The m6A “writer” consists of the catalytic subunit m6A-METTL complex (MAC) and the regulatory subunit m6A-METTL-associated complex (MACOM), the latter being essential for enzymatic activity. Deposition of m6A onto RNAs is achieved by the m6A methyltransferase complex (m6A writer), a large holocomplex of ~1000 kDa in size that contains methyltransferase-like 3 and 14 (METTL3/14), Wilms’ tumor 1-associated protein (WTAP), KIAA1429 (VIRMA), Zinc finger CCCH domain-containing protein 13 (ZC3H13), RNA binding motif protein 15/15 paralog (RBM15/15B), and E3 ubiquitin ligase CBLL1 (HAKAI). Here, we report the cryo-electron microscopy (cryo-EM) structures of MACOM at a 3.0-Å resolution, uncovering that WTAP and VIRMA form the core structure of MACOM and that ZC3H13 stretches the conformation by binding VIRMA. Our cryo-EM structure reveals that WTAP forms a homodimer, with each monomer consisting of four tandem helices (H1–H4/H1’–H4’ with coiled-coil interactions) and three linkers (L1–L3/L1’–L3’).

To understand the structural basis of the MACOM function, we determined the 3.0-Å resolution structures of the HWVZ and HWV complexes using single-particle cryo-EM analysis. To our surprise, in the cryo-EM structure of the HWVZ complex, only three components (WTAP, VIRMA, and ZC3H13) can be found, while HAKAI is missing, although it is present in the SDS-PAGE analysis, indicating the high flexibility of HAKAI. Human WTAP (residues 64–247), VIRMA (residues 334–1585), and ZC3H13 (residues 1492–1643) form a compact structure shaped like a “warhorse” that represents the core of human MACOM. Unlike WTAP and VIRMA that form saddle- and horse-like conformations, respectively, the C-terminal fragment of ZC3H13 is only one-tenth of its full length and contains eight α-helices, but it does not exhibit a rigid conformation. Instead, it attaches to the Belly, Chest, and Neck domains of VIRMA and functions like a barding to protect the horse body (Supplementary informaiton, Video S1). Therefore, this fragment of ZC3H13 is called the Barding domain. The Barding domain of ZC3H13 has a strong interaction with VIRMA, and the interface is ~4435 Å2, involving seven salt bridges and 19 hydrogen bonds. In contrast, the interaction between the Barding domain and WTAP is weak, with an interface area of ~256 Å2 in which highly conserved residues R1512 and F1521 of the first α-helix of the Barding domain form salt bridges and hydrophobic interactions with D206 and F207 in H4 of WTAP-a, respectively. Our structural study shows that ZC3H13 uses its C-terminal Barding domain to interact with VIRMA and induce the conformational change of MACOM.

> MAVDSAMELLFLDTFKHPSAEQSSHIDVVRFPCVVYINEVRVIPPGVRAHSSLPDNRAYGETSPHTFQLDLFFNNVSKPSAPVFDRLGSLEYDENTSIIFRPNSKVNTDGLVLRGWYNCLTLAIYGSVDRVISHDRDSPPPPPPPPPPPQPQPSLKRNPKHADGEKEDQFNGSPPRPQPRGPRTPPGPPPPDDDEDDPVPLPVSGDKEEDAPHREDYFEPISPDRNSVPQEGQYSDEGEVEEEQQEEGEEDEDDVDVEEEEDEDEDDRRTVDSIPEEEEEDEEEEGEEDEEGEGDDGYEQISSDEDGIADLERETFKYPNFDVEYTAEDLASVPPMTYDPYDRELVPLLYFSCPYKTTFEIEISRMKDQGPDKENSGAIEASVKLTELLDLYREDRGAKWVTALEEIPSLIIKGLSYLQLKNTKQDSLGQLVDWTMQALNLQVALRQPIALNVRQLKAGTKLVSSLAECGAQGVTGLLQAGVISGLFELLFADHVSSSLKLNAFKALDSVISMTEGMEAFLRGRQNEKSGYQKLLELILLDQTVRVVTAGSAILQKCHFYEVLSEIKRLGDHLAEKTSSLPNHSEPDHDTDAGLERTNPEYENEVEASMDMDLLESSNISEGEIERLINLLEEVFHLMETAPHTMIQQPVKSFPTMARITGPPERDDPYPVLFRYLHSHHFLELVTLLLSIPVTSAHPGVLQATKDVLKFLAQSQKGLLFFMSEYEATNLLIRALCHFYDQDEEEGLQSDGVIDDAFALWLQDSTQTLQCITELFSHFQRCTASEETDHSDLLGTLHNLYLITFNPVGRSAVGHVFSLEKNLQSLITLMEYYSKEALGDSKSKKSVAYNYACILILVVVQSSSDVQMLEQHAASLLKLCKADENNAKLQELGKWLEPLKNLRFEINCIPNLIEYVKQNIDNLMTPEGVGLTTALRVLCNVACPPPPVEGQQKDLKWNLAVIQLFSAEGMDTFIRVLQKLNSILTQPWRLHVNMGTTLHRVTTISMARCTLTLLKTMLTELLRGGSFEFKDMRVPSALVTLHMLLCSIPLSGRLDSDEQKIQNDIIDILLTFTQGVNEKLTISEETLANNTWSLMLKEVLSSILKVPEGFFSGLILLSELLPLPLPMQTTQVIEPHDISVALNTRKLWSMHLHVQAKLLQEIVRSFSGTTCQPIQHMLRRICVQLCDLASPTALLIMRTVLDLIVEDLQSTSEDKEKQYTSQTTRLLALLDALASHKACKLAILHLINGTIKGDERYAEIFQDLLALVRSPGDSVIRQQCVEYVTSILQSLCDQDIALILPSSSEGSISELEQLSNSLPNKELMTSICDCLLATLANSESSYNCLLTCVRTMMFLAEHDYGLFHLKSSLRKNSSALHSLLKRVVSTFSKDTGELASSFLEFMRQILNSDTIGCCGDDNGLMEVEGAHTSRTMSINAAELKQLLQSKEESPENLFLELEKLVLEHSKDDDNLDSLLDSVVGLKQMLESSGDPLPLSDQDVEPVLSAPESLQNLFNNRTAYVLADVMDDQLKSMWFTPFQAEEIDTDLDLVKVDLIELSEKCCSDFDLHSELERSFLSEPSSPGRTKTTKGFKLGKHKHETFITSSGKSEYIEPAKRAHVVPPPRGRGRGGFGQGIRPHDIFRQRKQNTSRPPSMHVDDFVAAESKEVVPQDGIPPPKRPLKVSQKISSRGGFSGNRGGRGAFHSQNRFFTPPASKGNYSRREGTRGSSWSAQNTPRGNYNESRGGQSNFNRGPLPPLRPLSSTGYRPSPRDRASRGRGGLGPSWASANSGSGGSRGKFVSGGSGRGRHVRSFTR;> PVATATATTVPATLAATTAAAATSFSTSAITISTSATPTNTTNNTFANEDSHRKCHRTRVEKVETPHVTIEDAQHRKPMDQKRSSSLGSNRSNRSHTSGRLRSPSNDSAHRSGDDQSGRKRVLHSGSRDREKTKSLEITGERKSRIDQLKRGEPSRSTSSDRQDSRSHSSRRSSPESDRQVHSRSGSFDSRDRLQERDRYEHDRERERERRDTRQREWDRDADKDWPRNRDRDRLRERERERERDKRRDLDRERERLISDSVERDRDRDRDRTFESSQIESVKRCEAKLEGEHERDLESTSRDSLALDKERMDKDLGSVQGFEETNKSERTESLEGDDESKLDDAHSLGSGAGEGYEPISDDELDEILAGDAEKREDQQDEEKMPDPLDVIDVDWSGLMPKHPKEPREPGAALLKFTPGAVMLRVGISKKLAGSELFAKVKETCQRLLEKPKDADNLFEHELGALNMAALLRKEERASLLSNLGPCCKALCFRRDSAIRKQLVKNEKGTIKQAYTSAPMVDNELLRLSLRLFKRKTTCHAPGHEKTEDNKLSQSSIQQELCVS;>[2x]MTNEEPLPKKVRLSETDFKVMARDELILRWKQYEAYVQALEGKYTDLNSNDVTGLRESEEKLKQQQQESARRENILVMRLATKEQEMQECTTQIQYLKQVQQPSVAQLRSTMVDPAINLFFLKMKGELEQTKDKLEQAQNELSAWKFTPDSQTGKKLMAKCRMLIQENQELGRQLSQGRIAQLEAELALQKKYSEELKSSQDELNDFIIQLDEEVEGMQSTILVLQQQLKETRQQLAQYQQQQSQASAPSTSRTTASEPVEQSEATSKDCSRLTNGPSNGSSSRQRTSGSGFHREGNTTEDDFPSSPGNGNKSSNSSEERTGRGGSGYVNQLSAGYESVDSPTGSENSLTHQSNDTDSSHDPQEEKAVSGKGNRTVGSRHVQNGLDSSVNVQGSVL>[2x]GIDP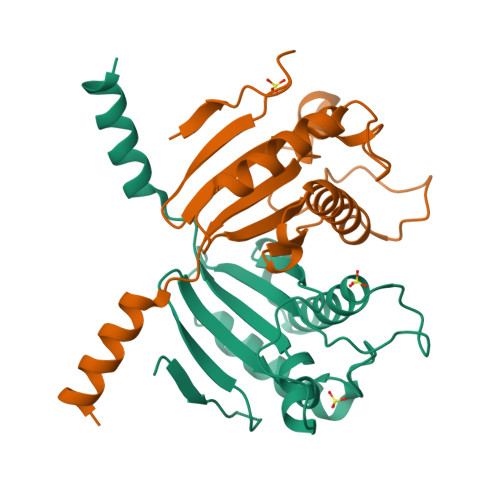FTEEQMASESSKPASQNTETKATIARKGEGSVLEQIDQGSILKLPSNLLFENATSDAINQDMMLYIERIAKIIQKLPKRVHINVRGFTDDTPLVKTRFKSHYELAANRAYRVMKVLIQYGVNPNQLSFSSYGSTNPIAPNDSLENRMKNNRVEIFFSTDANDLSKIHSILDNEFNPHKQQE2-AMINO-4-[1-CARBOXYMETHYL-CARBAMOYL)-2-HYDROXYMETHYLSULFANYL-ETHYLCARBAMOYL]-BUTYRIC ACID | C11 H19 N3 O7 S | 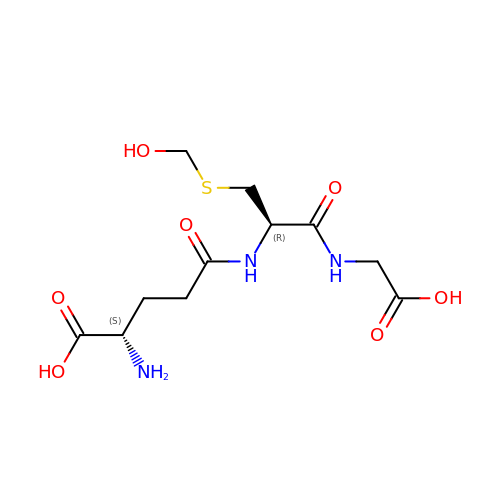PIUSLWSYOYFRFR-BQBZGAKWSA-N O-ACETYLSERINE | C5 H9 N O4 | 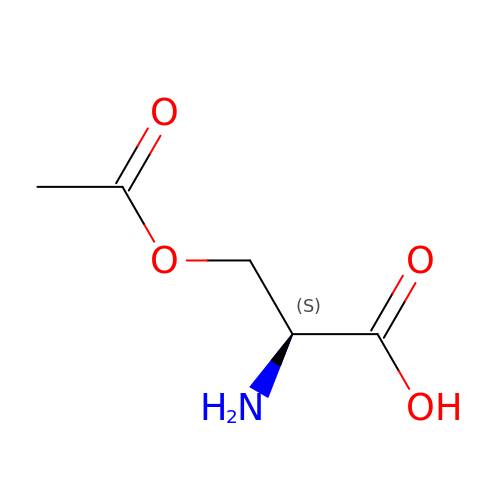VZXPDPZARILFQX-BYPYZUCNSA-N>GPMPGKKFVARVVEARAEDVGKRVVIIPKGIKVGDVVE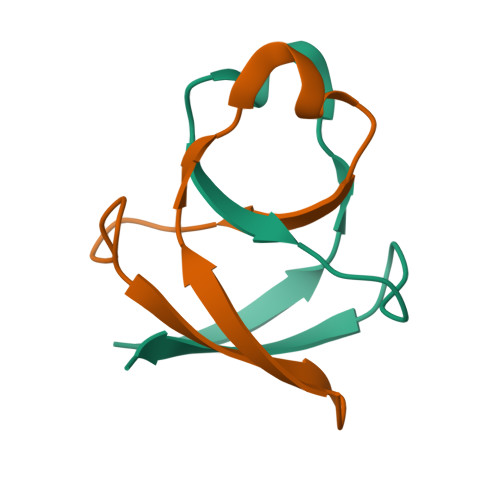VKKV[2x]>[2x]MKNFLETIEDMILIINREGRLLYA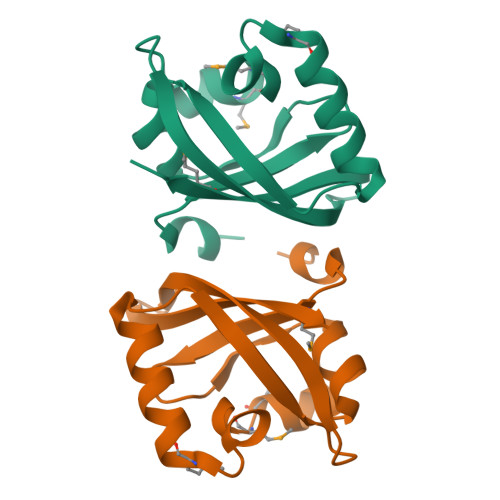NTAVPKKLGYTHEELMSMHILTITSAGKMAEGEKILAELFAGKKESLPLSLEKKEGTSIPAKARIWQGKWHNEPCLFAIIKDLSKEERASSPPFLEHHHHHH2-(2-BENZYL-6-HYDROXYADAMANTAN-2-YL)-1-(3-HYDROXYAZETIDIN-1-YL)ETHAN-1-ONE 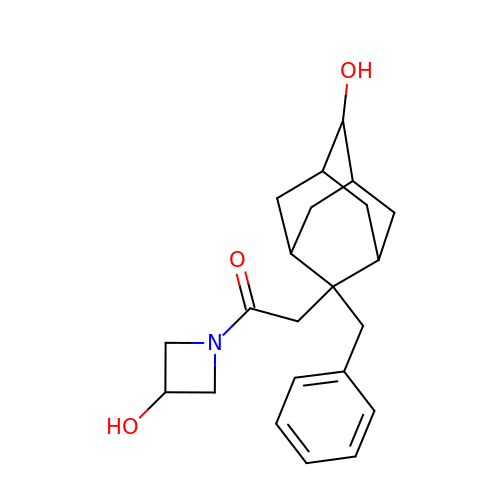| C22 H29 N O3 | TUDXSLUOQMCPRD-YORQRNKESA-N A monotopic alternative NADH dehydrogenase (Type II NADH dehydrogenase: NDH-2) catalyses the electron transfer from NADH to quinone via FAD or FMN without a proton-pumping activity, and functions as an initial enzyme, either in addition to or as an alternative to proton-pumping NADH dehydrogenase (complex I) in the respiratory chain of bacteria, archaea, and fungal and plant mitochondria. A series of studies has suggested that Ndi1, one of three NDH-2s from Saccharomyces cerevisiae, would be useful in replacement therapy for mitochondrial diseases caused by complex I dysfunction. We reported that the enzymatic reaction of yeast Ndi1 has a ping-pong mechanism, as is the case with NDH-2s from Mycobacterium tuberculosis and Yarrowia lipolytica. In this reaction mechanism, two substrates—NADH and ubiquinone—bind to the enzyme sequentially, but not at the same time.

A Lineweaver-Burk plot analyses indicated that stigmatellin is a competitive inhibitor whereas the others are mixed-type. There are no significant differences between the structures of the complexes, as indicated by root-mean-square deviations of 0.58–0.76 Å, which were calculated for 454–462 superimposed Cα positions.

> GVENSGAGPTSFKTMKVIDPQHSDKPNVLILGSGWGAISFLKHIDTKKYNVSIISPRSYFLFTPLLPSAPVGTVDEKSIIEPIVNFALKKKGNVTYYEAEATSINPDRNTVTIKSLSAVSQLYQPENHLGLHQAEPAEIKYDYLISAVGAEPNTFGIPGVTDYGHFLKEIPNSLEIRRTFAANLEKANLLPKGDPERRRLLSIVVVGGGPTGVEAAGELQDYVHQDLRKFLPALAEEVQIHLVEALPIVLNMFEKKLSSYAQSHLENTSIKVHLRTAVAKVEEKQLLAKTKHEDGKITEETIPYGTLIWATGNKARPVITDLFKKIPEQNSSKRGLAVNDFLQVKGSNNIFAIGDNAFAGLPPTAQVAHQEAEYLAKNFDKMAQIPNFQKNLSSRKDKIDLLFEENNFKPFKYNDLGALAYLGSERAIATIRSGKRTFYTGGGLMTFYLWRILYLSMILSARSRLKVFFDWIKLAFFKRDFFKGL;> TGVENSGAGPTSFKTMKVIDPQHSDKPNVLILGSGWGAISFLKHIDTKKYNVSIISPRSYFLFTPLLPSAPVGTVDEKSIIEPIVNFALKKKGNVTYYEAEATSINPDRNTVTIKSLSAVSQLYQPENHLGLHQAEPAEIKYDYLISAVGAEPNTFGIPGVTDYGHFLKEIPNSLEIRRTFAANLEKANLLPKGDPERRRLLSIVVVGGGPTGVEAAGELQDYVHQDLRKFLPALAEEVQIHLVEALPIVLNMFEKKLSSYAQSHLENTSIKVHLRTAVAKVEEKQLLAKTKHEDGKITEETIPYGTLIWATGNKARPVITDLFKKIPEQNSSKRGLAVNDFLQVKGSNNIFAIGDNAFAGLPPTAQVAHQEAEYLAKNFDKMAQIPNFQKNLSSRKDKIDLLFEENNFKPFKYNDLGALAYLGSERAIATIRSGKRTFYTGGGLMTFYLWRILYLSMILSARSRLKVFFDWIKLAFFKRDFFKGL(1R,2S)-cyclopentane-1,2-diol 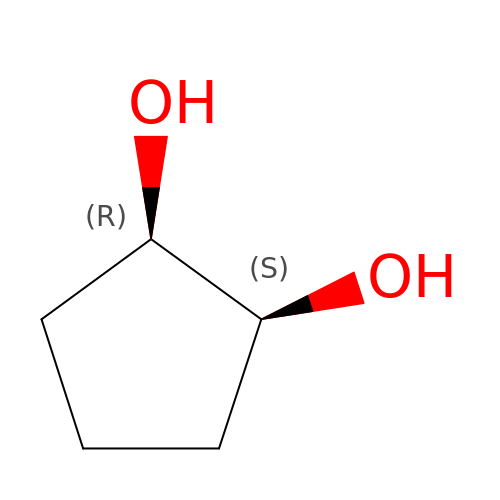| C5 H10 O2 | VCVOSERVUCJNPR-SYDPRGILSA-N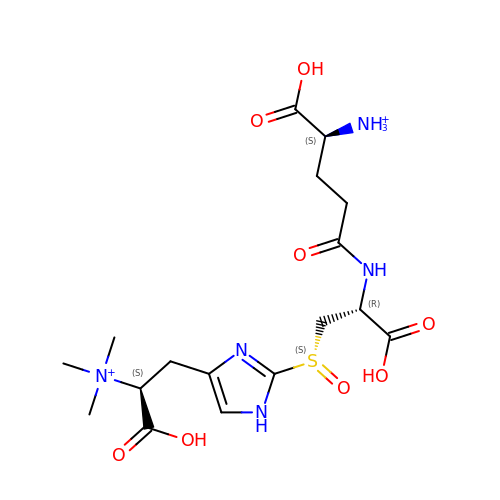(1S)-1-carboxy-4-({(1R)-1-carboxy-2-[(S)-{4-[(2S)-2-carboxy-2-(trimethylammonio)ethyl]-1H-imidazol-2-yl}sulfinyl]ethyl}amino)-4-oxobutan-1-aminium | C17 H29 N5 O8 S | SJHLSLUUWIBQNS-HBCRSHFUSA-P>EWSSTAITDRPTVNMLGGYYSQQQFLRNLDVRSNMASADQPSVMDEAYKEFVMQLASWDTRREFWLQTDYYKQRMVGNSKADA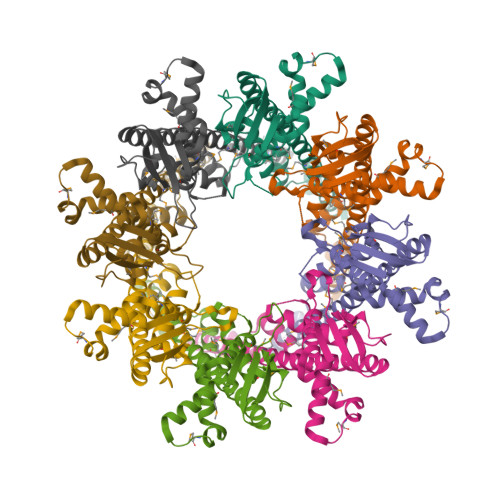ALLDEMINNIQFIPGDFTRAVNDSVKLIAETAPDANNLLRQYVAFASQRAASHLNDELKGAWAARTIQMKAQVKRQEEVAKAIYDRRMNSIEQALKIAEQHNISRSATDVPAEELPDSEMFLLGRPMLQARLENLQAVGPAFDLDYDQNRAMLNTLNVGPTLDPRFQTYRYLRTPEEPVKRD[8x]>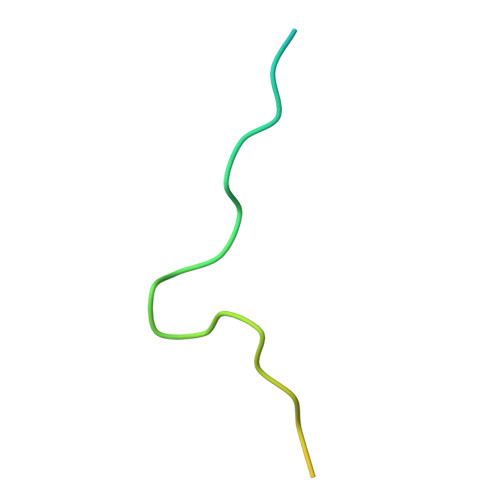 RLNTVTRVHQLMLEDAVTEREVLVTPGLEFLDDTTIPVGLMAQE> MKQYLELMQKVLDEGTQKNDRTGTGTLSIFGHQMRFNLQDGFPLVTTKRCHLRSIIHELLWFLQGDTNIAYLHENNVTIWDEWADENGDLGPVYGKQWRAWPTPDGRHIDQITTVLNQLKNDPDSRRIIVSAWNVGELDKMALAPCHAFFQFYVADGKLSCQLYQRTCDVFLGLPFNIASYALLVHMMAQQCDLEVGDFVWTGGDTHLYSNHMDQTHLQLS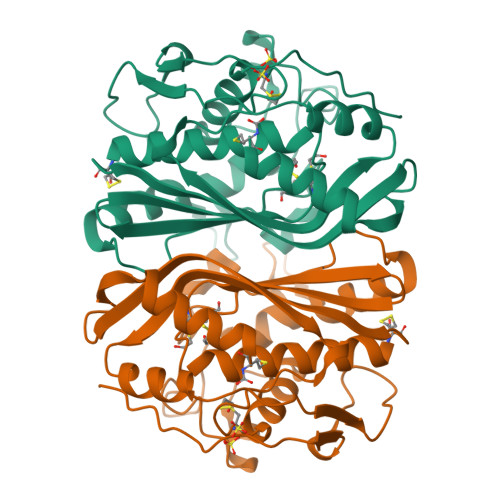REPRPLPKLIIKRKPESIFDYRFEDFEIEGYDPHPGIKAPVAI> MSEESQAFQRQLTALIGYDVTDVSNVHDDELEFTRRGLVTPRMAEVASRDPKLYAMHPWVTSKPLPEYLWKKIANNCIFIVIHRSTTSQTIKVSPDDTPGAILQSFFTKMAKKKSLMDIPESQSERDFVLRVCGRDEYLVGETPIKNFQWVRHCLKNGEEIHVVLDTPPDPALDEVRKEEWPLVDDCTGVTGYHEQLTIHGKDHESVFTVSLWDCDRKFRVKIRGIDIPVLPRNTDLTVFVEANIQHGQQVLCQRRTSPKPFTEEVLWNVWLEFSIKIKDLPKGALLNLQIYCGKAPALSSKASAESPSSESKGKVQLLYYVNLLLIDHRFLLRRGEYVLHMWQISGKGEDQGSFNADKLTSATNPDKENSMSISILLDNYCHPIALPKHQPTPDPEGDRVRAEMPNQLRKQLEAIIATDPLNPLTAEDKELLWHFRYESLKHPKAYPKLFSSVKWGQQEIVAKTYQLLARREVWDQSALDVGLTMQLLDCNFSDENVRAIAVQKLESLEDDDVLHYLLQLVQAVK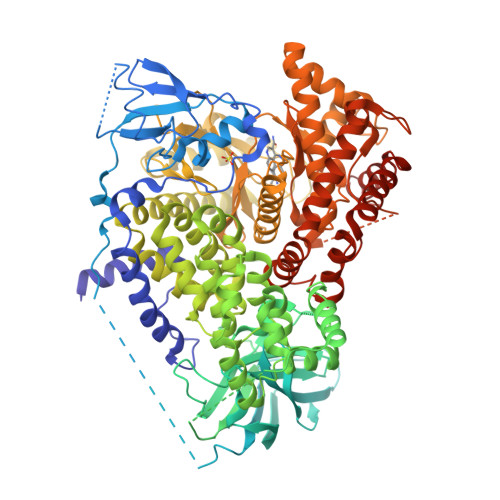FEPYHDSALARFLLKRGLRNKRIGHFLFWFLRSEIAQSRHYQQRFAVILEAYLRGCGTAMLHDFTQQVQVIEMLQKVTLDIKSLSAEKYDVSSQVISQLKQKLENLQNSQLPESFRVPYDPGLKAGALAIEKCKVMASKKKPLWLEFKCADPTALSNETIGIIFKHGDDLRQDMLILQILRIMESIWETESLDLCLLPYGCISTGDKIGMIEIVKDATTIAKIQQSTVGNTGAFKDEVLNHWLKEKSPTEEKFQAAVERFVYSCAGYCVATFVLGIGDRHNDNIMITETGNLFHIDFGHILGNYKSFLGINKERVPFVLTPDFLFVMGTSGKKTSPHFQKFQDICVKAYLALRHHTNLLIILFSMMLMTGMPQLTSKEDIEYIRDALTVGKNEEDAKKYFLDQIEVCRDKGWTVQFNWFLHLVLGIKQGEKHSAHHHHHH Here, we show that Paracoccus denitrificans assimilates ethylene glycol solely via NAD-dependent alcohol and aldehyde dehydrogenases. We report the functional and structural characterization of EtgB and EtgA, key enzymes encoded by this etg gene cluster. We hypothesized that the alcohol dehydrogenase EtgB can convert ethylene glycol into glycolaldehyde, which is subsequently further converted into glycolate by the aldehyde dehydrogenase EtgA. The cryo-EM structures of EtgA and EtgB, determined at 3.1 and 3.0 Å resolution, respectively, provide a detailed insight into the active site of these enzymes and a starting point for structure-guided mutagenesis.

The tetrameric EtgB is a class II zinc-dependent medium-chain alcohol dehydrogenase. We performed enzyme assays confirming that EtgB is indeed an alcohol dehydrogenase that utilizes NAD+ (NADH) as cofactor when converting alcohols to aldehydes (or vice versa). We found that this enzyme preferably accepts monoalcohols (ethanol, n-propanol, n-butanol) as substrates. The enzyme was found to catalyze the dehydrogenation of ethylene glycol, albeit with a kcat/Km value that is 300-fold lower than the kcat/Km for the conversion of ethanol. Nevertheless, when compared with NAD-dependent alcohol dehydrogenases characterized previously, EtgB shows favorable kinetic parameters with ethylene glycol as substrate. Therefore, we replaced the analogous Thr44 in EtgB with the smaller, isofunctional Ser to test for improved conversion of ethylene glycol and other diols. We also replaced His47 with Asn to probe the effect of this smaller amino acid on the active site and the proton-shuttling system. None of these mutations improved the catalytic efficiency for the dehydrogenation of ethylene glycol. However, EtgB H47N and especially EtgB T44S H47N showed improved catalytic efficiency with propylene glycol as substrate (ca. three-fold and ca. five-fold improved compared to EtgB WT, respectively).

>[4x]MGHHHHHHHHHHSSGHIEGRHNMAKTMKAAVVREFGKPLTIDEVPVPEPGPGMIQVRIQASGVCHTDLHAAEGDWPVKPNPPFIPGHEGVGFVSAVGAGVKHVKEGDRVGVPWLYTACGHCRHCLGGWETLCESQLNTGYSVNGGFADYVVADPNYVGHLPKNVDFLDIAPVLCAGVTVYKGLKVTDTKPGDWVVISGIGGLGHMAVQYAKAMGMNVAAVDIDDEKLALARKLGATVTVNAATEPDPAAAIRKQTDGGAQGVLVTAVGRKAFEQAIGMVARGGTVALNGLPPGDFPLDIFGMVLNGITVRGSIVGTRLDLQESLDFAGDGKVKATVHKAKLEDINNIFGQMHKGQIEGRMVLDMAG>[2x]SMKLQQLRYIWEVAHHDLNVSATAQ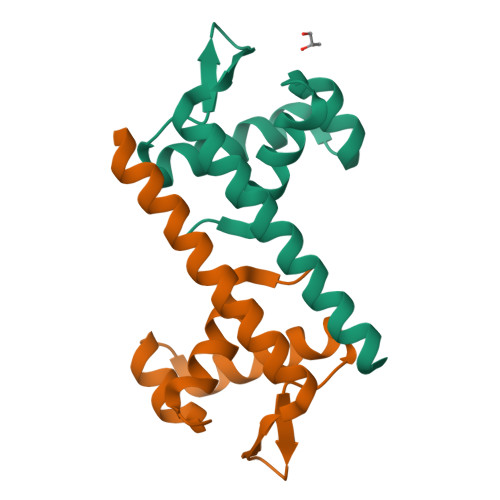SLYTSQPGISKQIRLLEDELGVEVFARSGKHLTRVTPAGERIIHTAGEILRKVESIKQIAQEFS> MANAVVDEETLEAMVYERSKAWSSKMADFASLEDGMEIDVAEFDNLFHGEDEDPDLDDVAKEAVEDNVPDEAKLEMGHINATSVTELTLILCANEDNEAKAEIEEILNQTVPVVEEHKRKWREAGLDRILDTFDEKQIEHHVGRWMRRHNSVYLEASPPKYLPPHHNSISDESDESMHSIDTARYIQQSRRRNAHMTNKNMTTIKMYRKHSHKRDELRAKYAYGDEQEHRHHMQAVLLRRRERERQLAYLASTPMQCVYSSGHHMRRKNLRKRRINSWMFDSASSSEEDTSFGGCDCHSCRRHYALSRSVYQSCPYGRGQREYHHRQMASRTM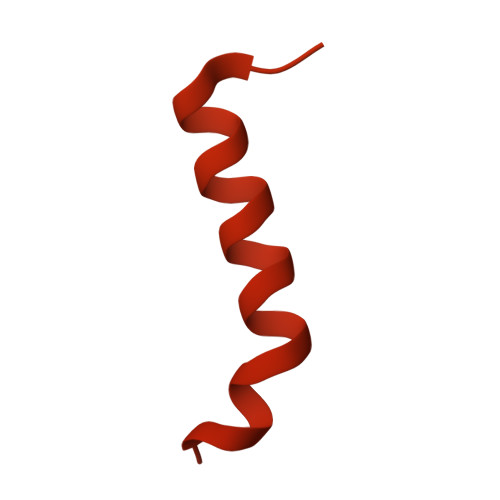HTMRRQHTFDMEMDLRPRLPENECSCCNSDRLCSNVIHIANSSTEEWVVENRSNHLTQETQEKTRKQKHQPMDARKVSHQPVCSKGHEQKPLSSKATSVSKLVLSKEKYMQMFDSESSDEDNALAKKGLLCCSDKKKGMTFPTPNAAGKITHPTSSAKKAIRKEARPNGLAQIQEEGPTATNSPIESTYLPVAHMKSVSIDGSSGTSATFESPAKKAPKRGIRETSPLNGNELQQLISTIPIADEKASSLMEKVDNCIGRESFDDRNKDFMHMENSSTKTAVEKSTKQKRVSGKKSEIPKSIITNNEILEKNSTETLSEKQVAAKAKKQSVRKTGATGKPSTSRLKKSEKTKTTSSVTSTSKLEQVREEESDVSSEVLAKPKPQCSTTASILKQGGDGASNSEDDLQIALAMSKATYKEEQQKRKKTKREPSNKQPQSPAEKSMTVFNNQSVACNSTALANDTACYRVLPKRRGVKRAAAVSTTEEKTATNSSSSPTSSLEEMGSPTGGDPDCTVVTSTTGCEPPASERQEIPATIKITKRGILLHSPSAPEGASFTLTEQGLGKIIGERWARKYLKYHIGSRSFDSRHSVYYQPTPQLAAALSAPQDAQNIGNISGSSASDDDIFEQINRYGTVYSILENNSGDK> MHHHHHHMLSVDDCFGMGRSAYNEGDYYHTVLWMEQVLKQLDAGEEATTTKSQVLDYLSYAVFQLGDLHRALELTRRLLSLDPSHERAGGNLRYFEQLLEEE;> PPPPPPPP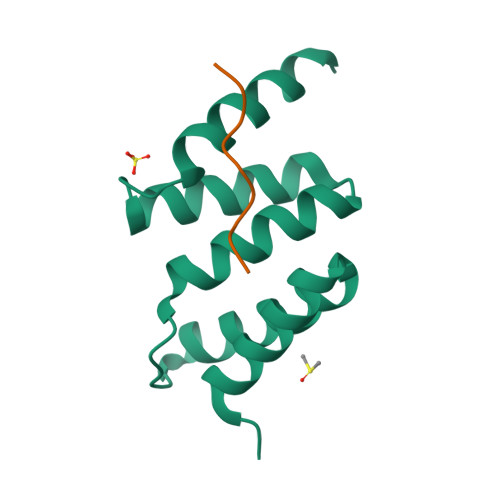P3-amino-2-benzoyl-4-methylthieno[2,3-b]pyridin-6-ol | C15 H12 N2 O2 S | 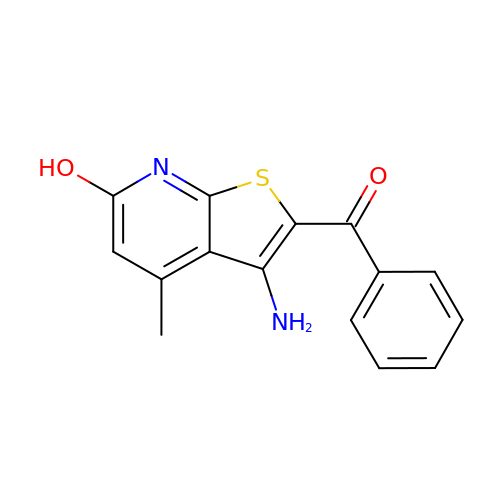PNCPOBGZUHFDDF-UHFFFAOYSA-N> FVQWNSRYSYNQLKNKDSLIMFLVEIFRSLFVSNCIDKNIDNVLLSIEEMFIDHYYNPQHSRLKYLIDDVGIFFTKLPITKAFHTYNKKYRITKRLYAPPTFNEVRHILNLAQILSLEEGLDLLTFDANETLYPDGHDFNDEVLASYISCLLKKMNIAIVTAASYNNDAEKYQKRLENLLKYFSKHNIKDGSYKNFYVMGGESNYLFKCNEE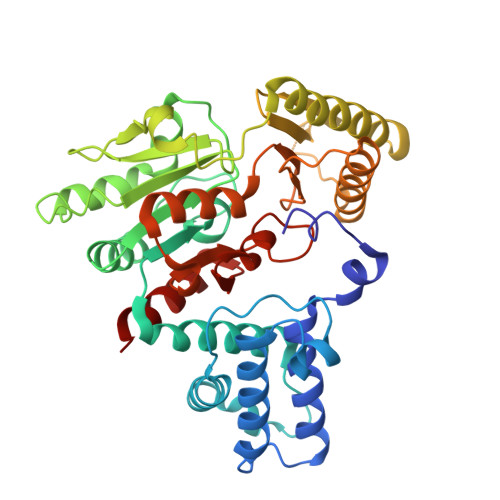ATLYSVPENEWRHYKKFVDYDTVQEILNISEKCLEKVIKDFGLCAQIQRKEKSIGLVPNKIPSLNIKNEQKNYMIKYEVLEEAVIRIKKEIIKNKITAPYCAFNGGQDLWVDVGNKAEGLLILQKLLKIQKKKCCHIGDQFLHSGNDFPTRFCSLTLWVSNPQETKACLKSIMHLN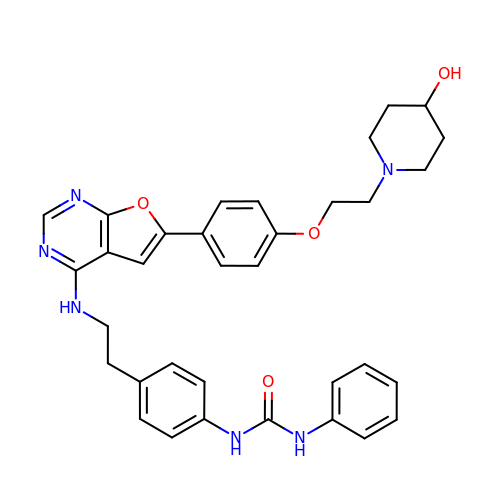1-(4-{2-[(6-{4-[2-(4-hydroxypiperidin-1-yl)ethoxy]phenyl}furo[2,3-d]pyrimidin-4-yl)amino]ethyl}phenyl)-3-phenylurea | C34 H36 N6 O4 | WEVRAOPLGYJTLY-UHFFFAOYSA-N>[2x]GGGAUACAGGACUGGCGGAUUAGUGGGAA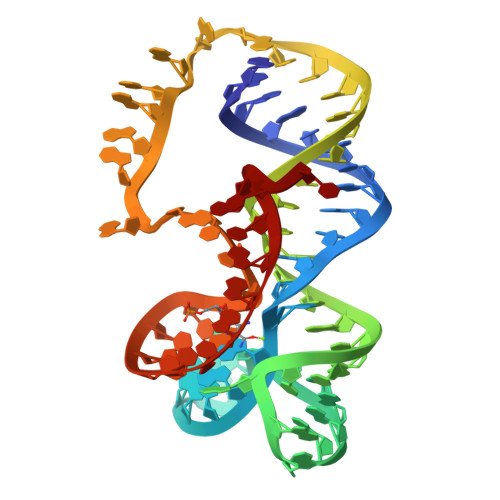ACCACGUGGACUGUAUCCGAAAAAAAGCCGACCGCCUGGGCAUC>[6x]ETLVRPKPLLLKLLKSVGAQKDTYTMKEVLFYLGQYI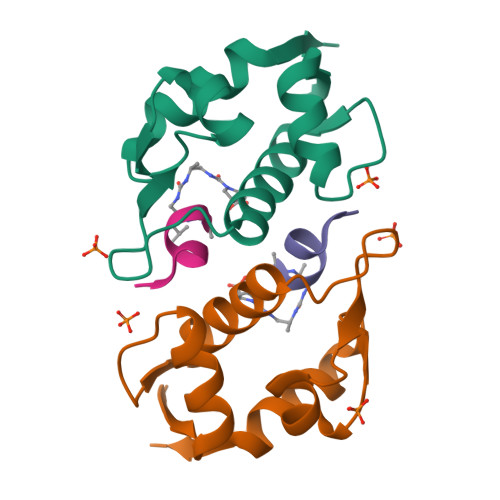MTKRLYDEKQQHIVYCSNDLLGDLFGAPSFSVKEHRKIYTMIYRNLVVV;>[6x]TSFAEYWAXXP>GPGSVDSVLFGSLRGHVVGLRYYTGVVNNNEMVALQRDPNNPYDKNAIKVNNVNGNQVGHLKKELAGALAYIMDNKLAQIE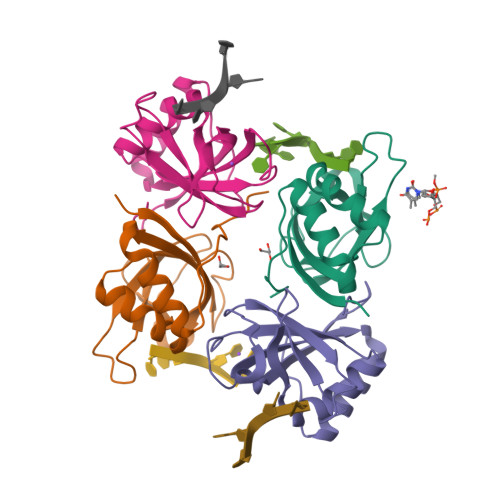GVVPFGANNAFTMPLHMTFWGKEENRKAVSDQLKKHGFKLGPAPKTLGF[4x]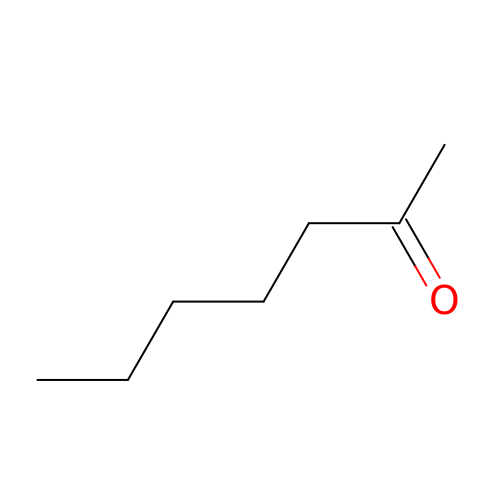heptan-2-one | C7 H14 O | CATSNJVOTSVZJV-UHFFFAOYSA-N> TSAKSNLMLILLGLQMKEISNSDLYKLKEVRSVVTSLASFLFQQQNVGVMKSFDSLEKEAFRDLVNRLVSQGLIGLKDKTSETFDLLPLKNLFEYAEKRISVLMKLQCYTGTVQLSHVQEKLHLPYITTNGIVDVFKECLKRTKKQYPEVLKNWWIDLDPKNGME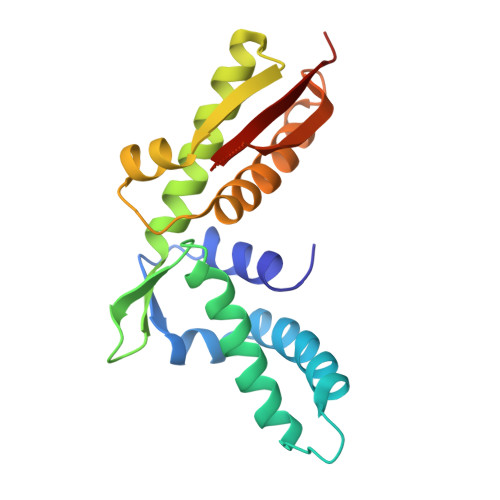DQNSGILLHLEYAA>NEEFRPEMLQGKKVIVTGASKGIGREMAYHLAKMGAHVVVTARSKETLQKVVSHCLELGAASAHYIAGTMEDMTFAEQFVAQAGKLMGGLDMLILNHITNTSLNLFHDDIHHVRKSMEVNFLSYVVLTVAALPMLKQSNGSIVVVSSLAGKVAYPLVAAYSASKFALDGFFSSIRKEYSVSRVNVSITLCVLGLIDTETAMKAVSGIVHMQAA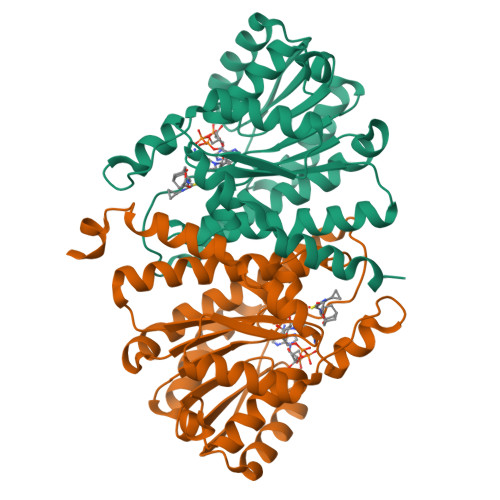PKEECALEIIKGGALRQEEVYYDSSRWTTLLIRNPSRKILEELYSTSYNMDRFINK[4x]> GMATMEELQREINAHEGQLVIARQKVRDAEKQYEKDPDELNKRTLTDREGVAVSIQAKIDELKRQL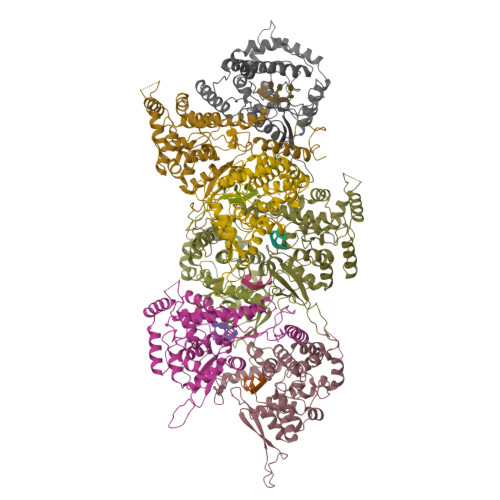ADRIATGKNLGKEQDPTGVEPGDHLKERSMLSYGNVLDLNHLDIDEPTGQTADWLSIIVYLTSFVVPILLKALYMLTTRGRQTTKDNKGTRIRFKDDSSFEDVNGIRKPKHLYVSLPNAQSSMKAEEITPGRYRTAVCGLYPAQIKARQMISPVMSVIGFLALAKDWSDRIEQWLIEPCKLLPDTAAVSLLGGPATNRDYLRQRQVALGNMETKESKAIRQHAEAAGCSMIEDIESPSSIWVFAGAPDRCPPTCLFIAGIAELGAFFSILQDMRNTIMASKTVGTSEEKLRKKSSFYQSYLRRTQSMGIQLGQRIIVLFMVAWGKEAVDNFHLGDDMDPELRTLAQSLIDVKVKEISNQEPLKL>[2x]SMNENYLQAVKDSAKSQYASLRESYKSITGKTESADELPDHDAEVLDSIMDRLHEPLYEKDTFDPNEVLAENKQLYEEFLLQEISEPKVDNLVRSGDPLAGKAKGTILSLVRNSDLEDIISSIQQLEEEYNKNFGYPYTFLNDEEFTDEFKDGIKSILPKDRVVEFGTIGPDNWNMPDSIDRERYDQEMDKMSKENIQYAEVESYHNMCRFYSKEFYHHPLLSKYKY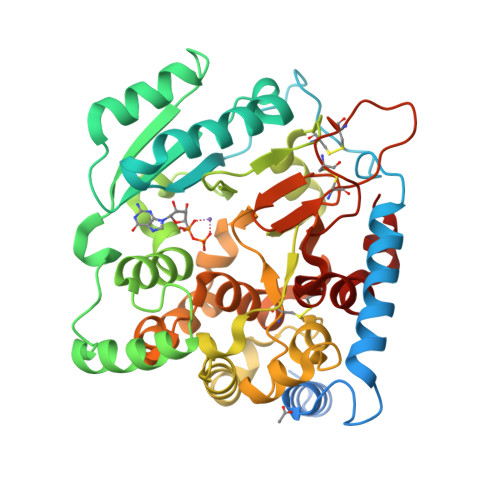VWRLEPNVNFYCKINYDVFQFMNKNDKIYGFVLNLYDSPQTIETLWTSTMDFVEEHPNYLNVNGAFAWLKDNSQNPKNYDYTQGYSTCHFWTNFEIVDLDFLRSEPYEKYMQYLEEKGGFYYERWGDAPVRSLALALFADKSSIHWFRDIGYHHTPYTNCPTCPADSDRCNGNCVPGKFTPWSDLDNQNCQATWIRHSMSEEELEMY BENZENE-1,2,3-TRIOL 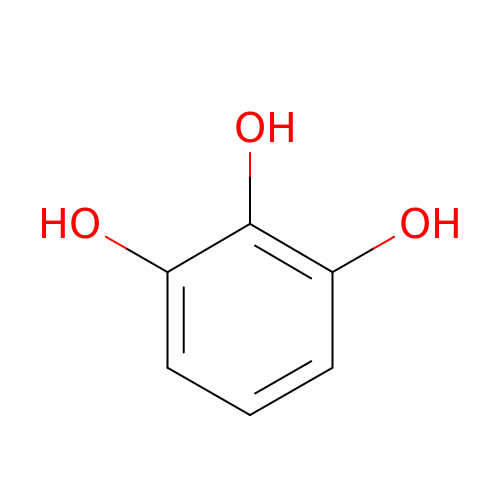| C6 H6 O3 | WQGWDDDVZFFDIG-UHFFFAOYSA-N>[4x]SPLAAYEVDDSTGYLTSDVGGPIQDQTSLKAGIRGPTLLEDFMFRQKIQHFDHERVPERAVHARGAGAHGTFTSYADWSNITAASFLNATGKQTPVFVRFSTVAGSRGSADTARDVHGFATRFYTDEGNFDIVGNNIPVFFIQDAIQFPDLIHSVKPRPDNEIPQAATAHDSAWDFFSQQPSTMHTLFWAMSGHGIPRSYRHMDGFGVHTFRFVKDDGSSKLIKWHFKSRQGKASLVWEEAQVLSGKNADFHRQDLWDAIESGNGPEWDVCVQIVDESQAQAFGFDLLDPTKIIPFEYAPLTKLGLLKLDRNPTNYFAETEQVMFQPGHIVRGIDFTEDPLLQGRLFSYLDTQLNRNGGPNFEQLPINMPRVPIHNNNRDGAGQMFIHRNKYPYTPNTLNSGYPRQANQNAGRGFFTAPGRTASGALVREVSPTFNDHWSQPRLFFNSLTPVEQQFLVNAMRFEISLVKSEEVKKNVLTQLNRVSHDVAVRVAAAIGLGAPDADDTYYHNNKTAGVSIVGSGPLPTIKTLRVGILATTSESSALDQAAQLRTRLEKDGLVVTVVAETLREGVDQTYSTADATGFDGVVVVDGAAALFASTASSPLFPTGRPLQIFVDAYRWGKPVGVCGGKSSEVLDAADVPEDGDGVYSEESVDMFVEEFEKGLATFRFTDRFALDS

Catalases (hydrogen-peroxide:hydrogen-peroxide oxido­reductases; EC 1.11.1.6) are redox enzymes that are responsible for the dismutation of hydrogen peroxide into water and molecular oxygen. The structures reveal a homotetrameric enzyme in which each of the four active sites consists of a pentacoordinated iron protoporphyrin IX prosthetic group with a tyrosin­ate axial ligand. The heme is deeply buried inside the protein, with a complex network of channels providing access to the exterior. We have previously shown that in addition to catalase activity, the catalase from S. thermophilum (CATPO) possesses a promiscuous phenolic oxidase activity in the absence of hydrogen peroxide.

We therefore generated a series of site-directed mutants around the putative 3TR/catechol binding pocket to further test this hypothesis. The residues Pro158, His246, Gln293, Ile313, Ile314, Glu316, Leu321 and Val536 surround the 3TR binding pocket and are structurally homologous to the residues that bind NADPH in the mammalian catalases. Specifically, the variants P158W, H246W, Q293W, I313F, I314F, E316F, E316H, L321A, V536A and V536W were constructed. The bulky phenylalanine side chain of the E316F variant is oriented away from the entrance to the lateral channel and putative oxidase substrate-binding pocket and thus it is not surprising that mutations at this position show minimal effect on the oxidase activity. The catechol oxidase activities of the H246W, I314F, L321A and V536W variants were noticeably reduced (50–92%) with respect to the wild-type enzyme, whereas the E316F, E316H, I313F and V536A variants of CATPO had little effect on the oxidase activity.> KLGDICFSLRYVPTAGKLTVVILEAKNLKKMDVGGLSDP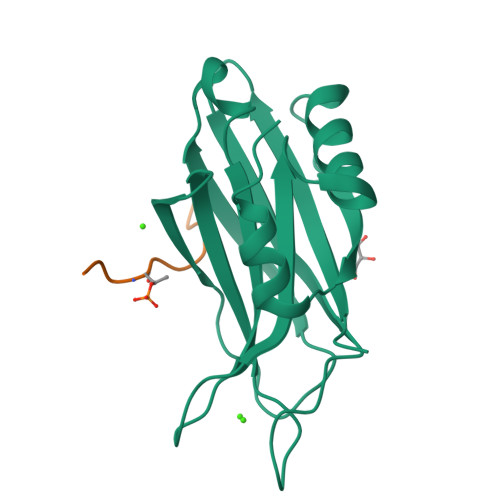YVKIHLMQNGKRLKKKKTTIKKNTLNPYYNESFSFEVPFEQIQKVQVVVTVLDYDKIGKNDAIGKVFVGYNSTGAELRHWSDMLANPRRPIAQWHTLQVEEEVDAMLAVKK;> SDATEGHDED>[2x]MNNRRFDC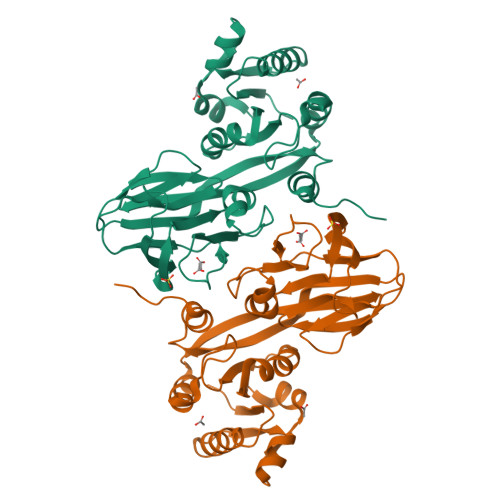IGIVGHPRHPAALATHEILYHWLKARGYAVMVEQQIAHDLNLTDAITGSLADIGQKADLAVVVGGDGNMLGAARVLARYDIKVIGVNRGNLGFLTDLDPDNALQQLSDVLEGEYLSEQRFLLETHVRRTNQQSRISTAINEVVLHPGKVAHMIEFEVYIDDRFAFSQRSDGLIIATPTGSTAYSLSAGGPILTPTLDAIVLVPMFPHTLTARPLVISSSSTIRLKFSHITSDLEISCDSQIALPIQEGEEVLIRRSDFHLNLIHPKDYSYFNTLSTKLGWSKKLFENLYFHHHHHH>[2x]GSMENTDVFLGLHDFLERMRKPSAGDFVKSIKSFIVSFSNNAPDPEKDCAMVQEFFS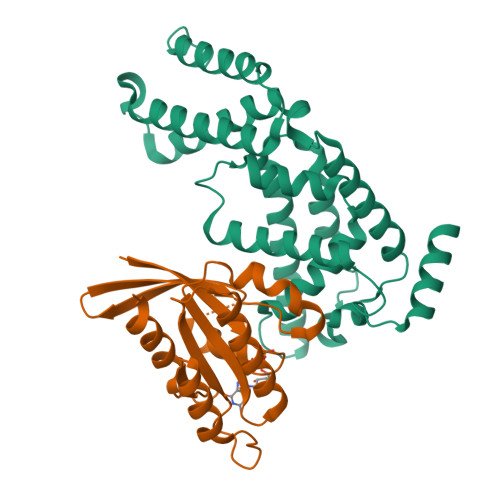KMEAAFRAHPLWSGCSEEELDSAGDGLEKYVMTKLFTRVFASNTEEVIADEKLFQKMSLVQQFISPENLDIQPTFQNESSWLLAQKELQKINMYKAPRDKLVCILNCCKVINNLLLNASIASNENAPGANEFLPVLIYVTIKANPPQLHSNLLYIQRYRRESKLVGEAAYFFTNILSAESFISNIDAKSISLDEAEFEKNMESARARISG;>GSMAAAGNKSINAKLVLLGDVGAGKSSLVLRFVKDQFVEFQESTIGAAFFSQTLAVNDATVKFEIWDTAGQERYHSLAPMYYRGAAAAIIVFDVTNQASFERAKKWVQELQAQGNPNMVMALAGNKSDLLDARKVTAEDAQTYAQENGLFFMETSAKTATNVKEIFYEIARRLPRVQPTEN[2x]> MGVFDRIRGALGRGLDVFRGDLPQVQPPAPQPAPAPAI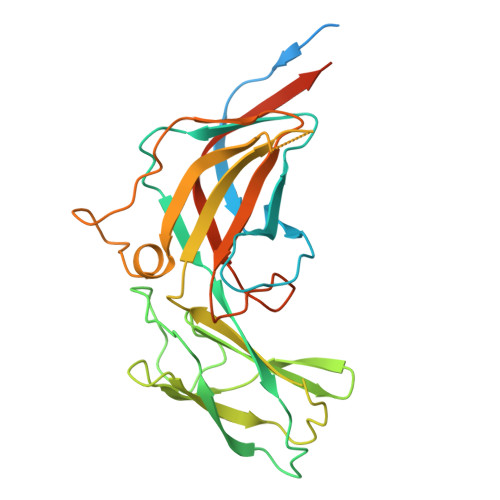TPAAVQVGGWGFAWIDNEDFSPTGLAWRSGEYFALAQMKTPETAHFRIAAQERRLRIYLRGQKVVNGRNLSDPDSRTVNLPFLMQTPQGAPTLPSTYHPDVAVWAKVGSTWQPCVITAINYSTGDVTFTEPAGVTASDGIEIYYVHGDGQFRLRVARDAGGVDDSAATVFNQSFSTMHSVDQNNVETMIAWPQQVELVPGTRLVLEVFTTQVPMVWNERSGHYIQIAAMGRRIEVLDKGGLQRLAELEARGGL>QAAKQLSQNFLLDLRLTDKIVRKAGNLTNAYVYEVGPGPGGITRSILNADVAELLVVEKDTRFIPGLQMLSDAAPGKLRIVHGDVLTFKVEKAFSESLKRPWEDDPPNVHIIGNLPFSVSTPLIIKWLENISCRDGPFVYGRTQMTLTFQKEVAERLAANTGSKQRSRLSVMAQYLCNVRHIFTIPGQAFVPKPEVDVGVVHFTPLIQPKIEQPFKLVEKVVQNVFQFRRKYCHRGLRMLFPEAQRLESTGRLLELADIDPTLRPRQLSISHFKSLCDVYRKMCDEDPQLFAYNFREELKRRKSKNEEKEEDDAENYRL[2x]

Mitochondrial transcription factor B1 (TFB1M) is a dimethyltransferase that maintains mitochondrial homeostasis by catalyzing dimethylation of two adjacent adenines located in helix45 (h45) of 12S rRNA. This m62A modification is indispensable for the assembly and maturation of human mitochondrial ribosomes. TFB1M was originally thought to serve as a transcription factor along with TFB2M but has instead been shown to be a dimethyltransferase with the main role of m62A modification of the 3′ end of mitochondrial 12S rRNA. To clarify the mechanism of m62A modification, we determined the crystal structures of a ternary complex of human (hs) TFB1M (hsTFB1M–h45–SAM) and a binary complex (hsTFB1M–h45) both at 3.0 Å resolution.

In this study, we report the first ternary complex structure of human TFB1M, SAM and h45. The structure of the ternary complex (hsTFB1M–h45–SAM) clearly showed how the substrate RNA, h45, interacts with hsTFB1M. In the structure, h45 folded into a hairpin structure capped with a typical four-nucleotide ‘GGAA’ tetraloop and was suspended from hsTFB1M, stretching across its N-terminal and C-terminal domains. As a typical SAM-dependent methyltransferase, hsTFB1M exhibited a conserved negatively-charged SAM-binding pocket surrounded by Glu85, Lys86, Asp111, Val112, Asn141, Leu142 and Val146, whose primary role was establishing hydrogen bonding and hydrophobic interactions. Two hydroxyl groups in the ribose moiety of SAM formed bidentate hydrogen bonds with the carboxyl group of Glu85. In the structure of the hsTFB1M–h45–SAM ternary complex, SAM lay in a conserved acidic pocket immediately adjacent to the m.937A pocket in order to present the SAM methyl group to one of the two N6H atoms in m.937A. Moreover, the active-site pocket, formed by the highly-conserved residues Gln35, Asn36, Asn141, Phe144 and Val225, could only accommodate one nucleotide of h45. Conversely, in our structure, h45 formed a stem loop and presented one adenine into the hsTFB1M active pocket. Based on the location of h45 in the 12S rRNA, we assume that the folding mode of h45 in the hsTFB1M–h45–SAM complex more accurately reflects the true enzymatic state. Thus, the process of m62A modification is possibly the same with m6A, during which the enzyme active center only accommodates one adenine and one SAM methyl group simultaneously.>[2x]SQTVHFQGNPVTVANSIPQAGSKAQTFTLVAKDLSDVTLGQFAGKRKVLNIFPSIDTGVCAAS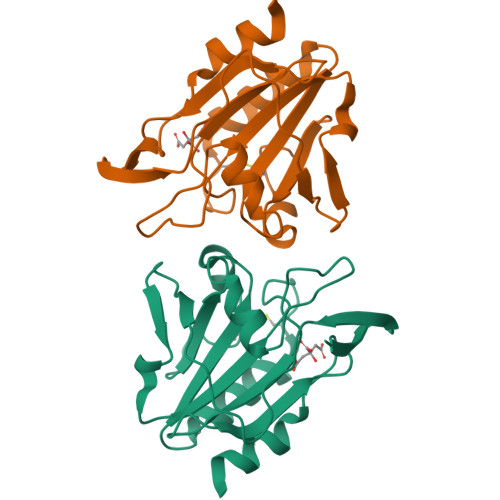VRKFNQLATEIDNTVVLCISADLPFAQSRFCGAEGLNNVITLSTFRNAEFLQAYGVAIADGPLKGLAARAVVVIDENDNVIFSQLVDEITTEPDYEAALAVLKA>GGADQKGPVFLKEPTNRIDFSNSTGAEIECKASGNPMPEIIWIRSDGTAVGDVPGLRQISSDGKLVFPPFRAEDYRQEVHAQVYACLARNQFGSIISRDVHVRAVVIQSYESEADNEYVIRGNSVVMKCEIPSYVADFVFVDLWLDSEGRNYYPNNAAETDGKYLVLPSGELHIREVGPEDGYKSYQCRTKHRLTGETRLSATKGRLVITEPVGSKAPTFATASKISSLLGSSSSDIVLLCQAQAFPVPYTRWYKFIEGTTRKQAVVLNDRVKQVSGTLIIKDAVVEDSGKYLCVVNN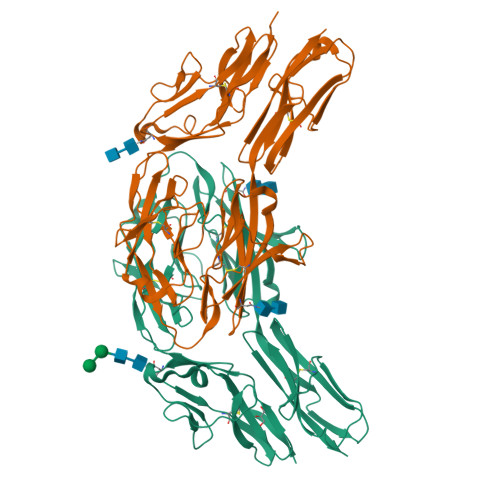SVGGESVETVLTVTAPLSAKIDPPTQTVDFGRPAVFTCQYTGNPIKTVSWMKDGKAIGHSEPVLRIESVKKEDKGMYQCFVRNDQESAEASAELKLGG[2x]N,N-dimethylmethanamine | C3 H9 N | 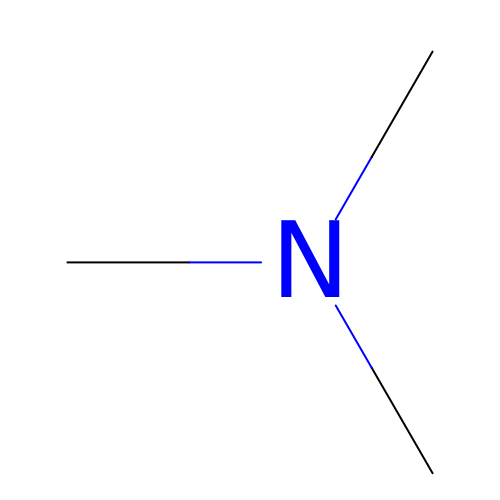GETQZCLCWQTVFV-UHFFFAOYSA-N>MTHQTHTIAESNNFIVLDKYIKAEPTGDSYQSESDLERELIQDLRNQGYEFISVKSQSAMLANVREQLQNLNGVVFNDSEWRRFTEQYLDNPSDGILDKTRKIHIDYICDFIFDDERLENIYLIDKKNLMRNKVQIIQQFEQAGSHANRYDVTILVNGLPLVQIELKKRGVAIREAFNQIHRYSKESFNSENSLFKYLQLFVISNGTDTRYFANTTKRDENSFDFTMNWAKSDNTLIKDLKDFTATCFQKHTLLNVLVNYSVFDSSQTLLVMRPYQIAATERILWKIKSSFTAKNWSKPESGGYIWHTTGSGKTLTSFKAARLATELDFIDKVFFVVDRKDLDYQTMKEYQRFSPDSVNGSENTAGLKRNLDKDDNKIIVTTIQKLNNLMKAESDLPVYNQQVVFIFDECHRSQFGEAQKNLKKKFKRYYQFGFTGTPIFPENALGSETTASVFGRELHSYVITDAIRDEKVLKFKVDYNDVRPQFKSLETETDEKKLSAAENQQAFLHPMRIQEITQYILNNFRQKTHRTFPGSKGFNAMLAVSSVDAAKAYYATFKRLQEEAANKSATYKPLRIATIFSFAANEEQNAIGEISDETFDTSAMDSSAKEFLDAAIREYNSHFKTNFSTDSNGFQNYYRDLAQRVKNQDIDLLIVVGMFLTGFDAPTLNTLFVDKNLRYHGLMQAFSRTNRIYDATKTFGNIVTFRDLERSTIDAITLFGDKNTKNVVLEKSYTEYMEGFTDAATGEAKRGFMTVVSELEQRFPDPTSIESEKEKKDFVKLFGEYLRAENILQNYDEFATLKALQQIDLSDPVAVEKFKAEHYVDDEKFAELQTIRLPADRKIQDYRSAYNDIRDWQRREKEAEKKEKSTTDWDDVVFEVDLLKSQEINLDYILGLIFEHNRQNKGKGEMIEEVKRLIRSSLGNRAKEGLVVDFIQQTNLDDLPDKASIIDAFFTFAQREQQREAEALIKEENLNEDAAKRYIRTSLKREYATENGTELNETLPKLSPLNPQYKTKKQAVFQKIVSFIEKFKGVGGKI[4x]

Type I RM enzymes house these activities in a multisubunit complex having ATP-dependent translocation activity that pulls thousands of duplex DNA base pairs through the stationary enzyme, eventually cleaving at random sites distant from the recognition site. Upon identification of an unmethylated specific DNA sequence, two HsdR motor subunits, which bear the endonuclease and ATP-dependent DNA translocation activities in the fully assembled DNA-HsdS-HsdM2-HsdR2 complex, start to translocate the duplex DNA toward the stationary enzyme from both directions, producing two extruded DNA loops flanking the enzyme complex. The X-ray crystal structure of the HsdR subunit with bound ATP from the Type I restriction enzyme of E. coli plasmid R124 revealed four structural and functional domains forming a planar array: one nuclease domain of PD-(E/D)xK type that houses three endonuclease active-site residues and a QxxxY motif common to the RecB-like nucleases; two RecA-like helicase domains of SF2 type that use ATP to translocate duplex DNA without unwinding; and a C-terminal α-helix-rich domain presumed to contact the HsdS-HsdM2 methylase. ATP bound between the two helicase domains was found unexpectedly to also contact Lys220 of the endonuclease domain, suggesting a means by which nuclease and translocation activities might communicate.

The three mutant HsdR subunits were crystallized with bound ATP, and their X-ray crystal structures were refined at 2.74 Å, 2.84 Å, and 2.99 Å for the Lys220Arg, Lys220Ala, and Lys220Glu mutants, respectively, guided by the higher-resolution structure of the WT HsdR-ATP complex (2.6 Å; 22). The overall structure of all four HsdRs in these crystals is the same, although the structures of the Lys220Arg and Lys220Ala mutants present only two molecules in the asymmetric unit whereas Lys220Glu has four; WT HsdR crystals have two molecules in the asymmetric unit. In the Lys220Glu mutant the loop is less defined than in the Lys220Ala structure, although main-chain atoms of residues 216–220 could be modeled. In the Lys220Ala and Lys220Glu structures, where the residue 220 sidechain does not form a hydrogen bond with ATP, the helix-like segment is rotated so as to bring the alpha carbon of Asn221 into the position of the alpha carbon of residue 220 in the WT and Lys220Arg structures. In these two structures the Asn221 sidechain points toward ATP and partially fills the space that in the other two structures is occupied by the sidechain of residue 220, but the Asn221 sidechain does not approach the ATP base edge closely enough to hydrogen bond as Lys220 or Arg220 can. Although the helix-like segment is also rotated in the Lys220Glu structure, the region preceding that segment is poorly defined in all four molecules of the asymmetric unit, and the Glu220 sidechain is not resolved. High mobility in this region may limit contact with the 180s loop.> 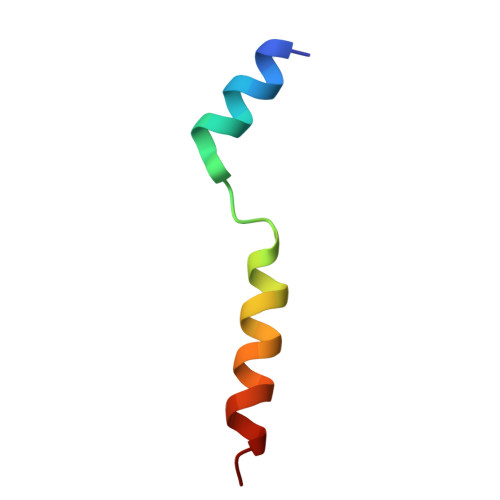GAMATNFLAHEKIWFDKFKYDDAERRFYEQMN>MPHDPGATRLLAISPHLDDAVLSFGAGLAQAAQDGANVLVYTVFAGAAQPPYSPAAQRMHTIWGLAPDDDAVLYRRKEDIAALDHLRVAHRHGRFLDS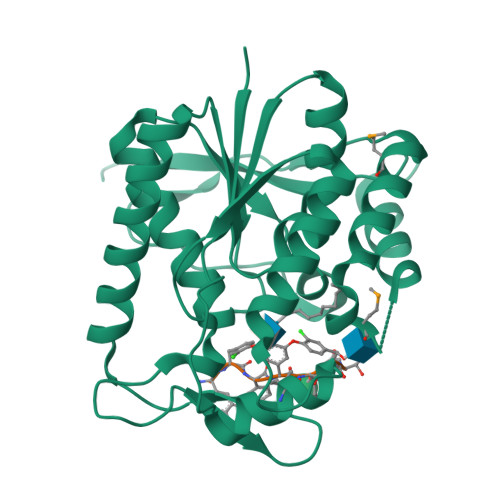IYRKLPDGRWLTAHVEGRQKLAVNDHSPDSDHDLVGEVADDIRSIIDEFDPTLVVTCAAIGEHPDNEATRDAALFATHEKNVPVRLWEDLPYAVFKSGAVELPQGFRLGSADVSSVKPEMRSQKFQAVERYSSQMVLLNGSENNLFDRLDEHARQNAPHGGYGETTWPVVRSDDS[4x]> MGPPSGKTYMGWWGHMGGPKQKGITSYAVS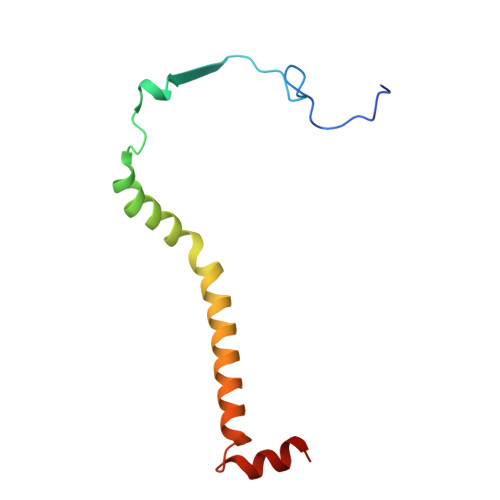PYAQKPLQGIFHNAVFNSFRRFKSQFLYVLIPAGIYWYWWKNGNEYNEFLYSKAGREELERVNV>GSHM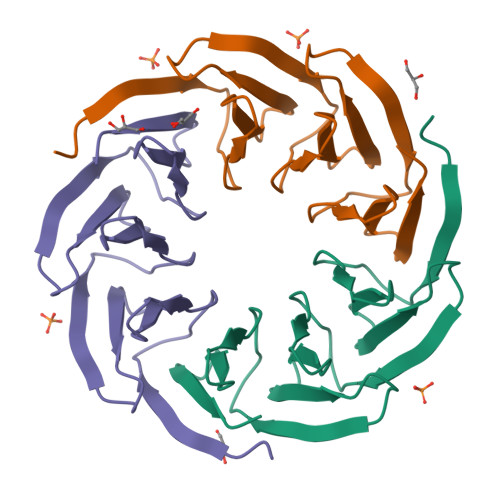DGTEKWRFKTGKAIEASPVIGEDGTIYVGSNDGHLYAINPDGTEKWRFKTGKAIEASPVIGEDGTIYVGSNDGHLYAINPDGTEKWRFKTGKAIEASPVIGEDGTIYVGSNDGHLYAINP[3x]>[2x]MAKDKEFQVLF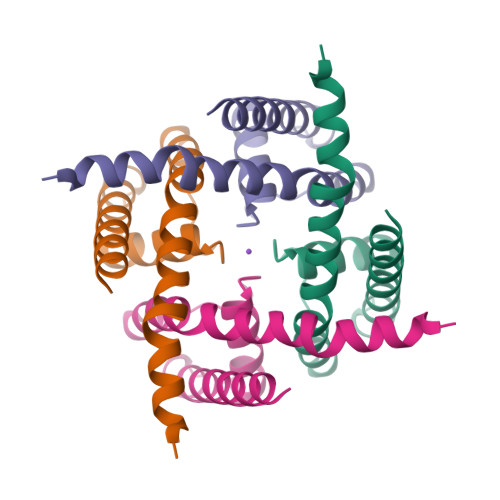VLTILTLISGTIFYSTVEGLRPIDALYFSVVTLTTVGFGDFSPQTDFGKIFTILYIFIGIGLVFGFIHKLAVNVQLPSILSNLVPR> GHMQETQAVEAGEKTVEQFVQALNKGDYNKAAEMTSKKAANKSALSEKEILDKYQNIYGAADVKGLQISNLKVDKKDDSTYSFSYKAKMNTSLGELKDLSYKGTLDRNDGQTTINWQPNLVFPEMEGNDKVSLTTQEAARGNIIDRNGEPLATTGKLKQLGVVPSKLGDGGEKTANIKAIASSFDLTEDAINQAISQSWVQPDYFVPLKIIDGATPELPAGATIQEVDGRYYPLGEAAAQLIGYVGDITAEDIDKNPELSSNGKIGRSGLEMAFDKDLRGTTGGKLSITDADGVEKKVLIEHEVQNGKDIKLTIDAKAQKTAFDSLGGKAGSTVATTPKTGDLLALASSPSYDPNKMTNGISQEDYKAYEENPEQPFISRFATGYAPGSTFKMITAAIGLDNGTIDPNEVLTINGLKWQKDSSWGSYQVTRVSDVSQVDLKTALIYSDNIYAAQETLKMGEKKFRTGLDKFIFGEDLDLPISMNPAQISNEDSFNSDILLADTGYG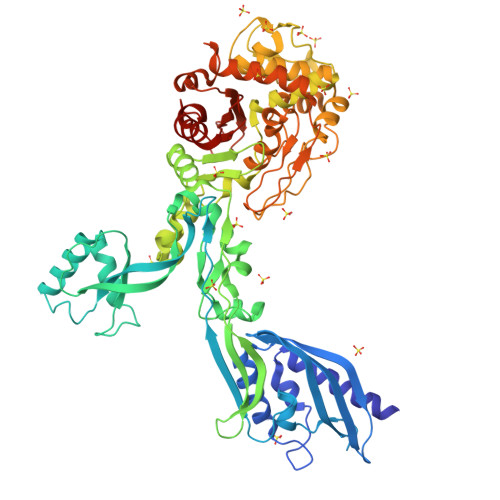QGELLINPIQQAAMYSVFANNGTLVYPKLIADKETKDKKNVIGETAVQTIVPDLREVVQDVNGTAHSLSALGIPLAAKTGTAEIKEKQDVKGKENSFLFAFNPDNQGYMMVSMLENKEDDDSATKRASELLQYLNQNYQ> GAMGSKCPTEEICKDFSNLPQCRKNVHERNNWLGSSVKNFSSDNKGV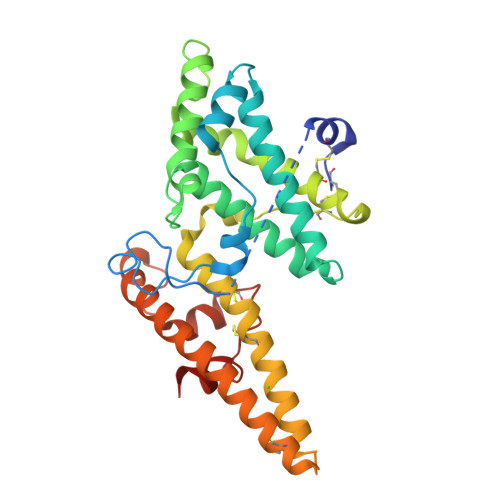LVPPRRQSLCLRITLQDFRTKKKKEGDFEKFIYSYASSEARKLRTIHNNNLEKAHQAIRYSFADIGNIIRGDDMMDTPTSKETITYLEKVLKIYNENNDKPKDAKKWWTENRHHVWEAMMCGYQSAQKDNQCTGYGNIDDIPQFLRWFREWGTYVCEESEKNMNTLKAVCFPKQPRTEANPALTVHENEMCSSTLKKYEEWYNKRKTEWTEQSIKYNNDKINYTDIKTLSPSEYLIEKCPECKCTKKNLQDVFELTFD> SLKITDDCINCDVCEPECPNGAI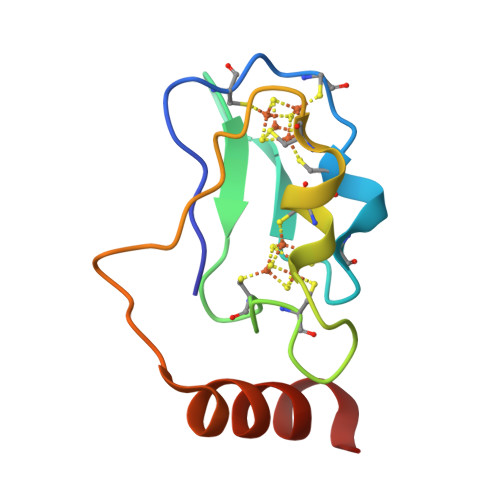SQGEEIYVIDPNLCTECVGHYDEPQCQQVCPVDCIPLDDANVESKDQLMEKYRKITGKA>GGSMSKSKVDNQFYSVEVGDSTFTVLKRYQNLKPIGSGAQGIVCAAYDAVLDRNVAIKKLSRPFQNQTHAKRAYR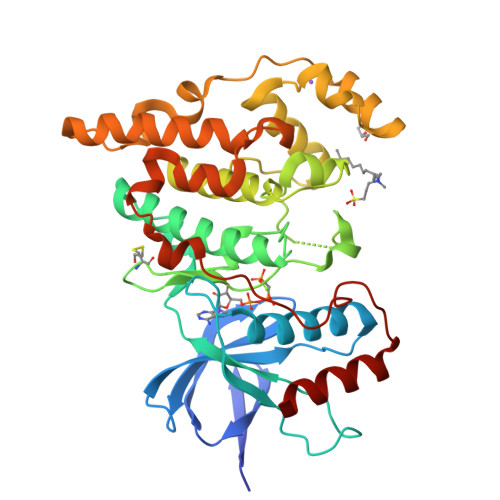ELVLMKCVNHKNIISLLNVFTPQKTLEEFQDVYLVMELMDANLCQVIQMELDHERMSYLLYQMLCGIKHLHSAGIIHRDLKPSNIVVKSDCTLKILDFGLARTAGTSFMMTPYVVTRYYRAPEVILGMGYKENVDIWSVGCIMGEMVRHKILFPGRDYIDQWNKVIEQLGTPCPEFMKKLQPTVRNYVENRPKYAGLTFPKLFPDSLFPADSEHNKLKASQARDLLSKMLVIDPAKRISVDDALQHPYINVWYDPAEVEAPPPQIYDKQLDEREHTIEEWKELIYKEVMNSE[2x]> MGPVTINNFNYNDPIDNNNIIMMEPPFARGTGRYYKAFKITDRIWIIPERYTFGYKPEDFNKSSGIFNRDVCEYYDPDYLNTNDKKNIFLQTMIKLFNRIKSKPLGEKLLEMIINGIPYLGDRRVPLEEFNTNIASVTVNKLISNPGEVERKKGIFANLIIFGPGPVLNENETIDIGIQNHFASREGFGGIMQMKFCPEYVSVFNNVQENKGASIFNRRGYFSDPALILMHQLIYVLHGLYGIKVDDLPIVPNEKKFFMQSTDAIQAEELYTFGGQDPSIITPSTDKSIYDKVLQNFRGIVDRLNKVLVCISDPNININIYKNKFKDKYKFVEDSEGKYSIDVESFDKLYKSLMFGFTETNIAENYKIKTRASYFSDSLPPVKIKNLLDNEIYTIEEGFNISDKDMEKEYRGQNKAINKQAYEEISKEHLAVYKIQMCKSVKAPGICIDVDNEDLFFIADKNSFSDDLSKNERIEYNTQSNYIENDFPINELILDTDLISKIELPSENTESLTDFNVDVPVYEKQPAIKKIFTDENTIFQYLYSQTFPLDIRDISLTSSFDDALLFSNKVYSFFSMDYIKTANKVVEAGLFAGWVKQIVNDFVIEANKSNTMDKIADISLIVPYIGLALNVGNETAKGNFENAFEIAGASILLEFIPELLIPVVGAFLLESYIDNKNKIIKTIDNALTKRNEKWSDMYGLIVAQWLSTVNTQFYTIKEGMYKALNYQAQALEEIIKYRYNIYSEKEKSNINIDFNDINSKLNEGINQAIDNINNFINGCSVSYLMKKMIPLAVEKLLDFDNTLKKNLLNYIDENKLYLIGSAEYEKSKVNKYLKTIMPFDLSIYTNDTILIEMFNKYNSEILNNIILNLRYKDNNLIDLSGYGAKVEVYDGVELNDKNQFKLTSSANSKIRVTQNQNIIFNSVFLDFSVSFWIRIPKYKNDGIQNYIHNEYTIINCMKNNSGWKISIRGNRIIWTLIDINGKTKSVFFEYNIREDISEYINRWFFVTITNNLNNAKIYINGKLESNTDIKDIREVIANGEIIFKLDGDIDRTQFIWMKYFSIFNTELSQSNIEERYKIQSYSEYLKDFWGNPLMYNKEYYMFNAGNKNSYIKLKKDSPVGEILTRSKYNQNSKYINYRDLYIGEKFIIRRKSNSQSINDDIVRKEDYIYLDFFNLNQEWRVYTYKYFKKEEEKLFLAPISDSDEFYNTIQIKEYDEQPTYSCQLLFKKDEESTDEIGLIGIHRFYESGIVFEEYKDYFCISKWYLKEVKRKPYNLKLGCNWQFIPKDEGWTEHHHHHHHHHH;> MNINDNLSINSPVDNKNVVVVRARKTDTVFKAFK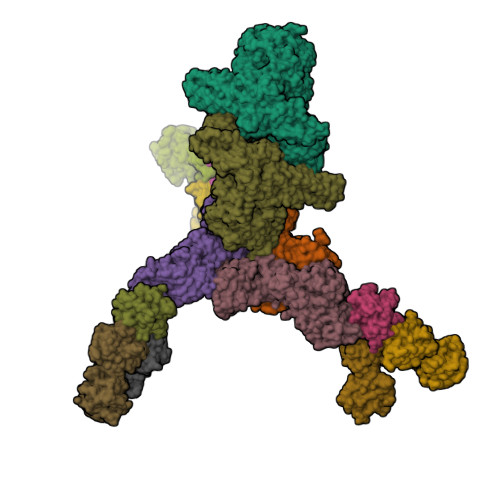VAPNIWVAPERYYGESLSIDEEYKVDGGIYDSNFLSQDSEKDKFLQAIITLLKRINSTNAGEKLLSLISTAIPFPYGYIGGGYYAPNMITFGSAPKSNKKLNSLISSTIPFPYAGYRETNYLSSEDNKSFYASNIVIFGPGANIVENNTVFYKKEDAENGMGTMTEIWFQPFLTYKYDEFYIDPAIELIKCLIKSLYFLYGIKPSDDLVIPYRLRSELENIEYSQLNIVDLLVSGGIDPKFINTDPYWFTDNYFSNAKKVFEDHRNIYETQIEGNNAIGNDIKLRLKQKFRININDIWELNLNYFSKEFSIMMPDRFNNALKHFYRKQYYKIDYPENYSINGFVNGQINVQLSLSDRNQDIINKPEEIINLLNGNNVSLMRSNIYGDGLKSTVDDFYSNYKIPYNRAYEYHFNNSNDSSLDNVNIGVIDNIPEIIDVNPYKENCDKFSPVQKITSTREINTNIPWPINYLQAQNTNNEKFSLSSDFVEVVSSKDKSLVYSFLSNVMFYLDSIKDNSPIDTDKKYYLWLREIFRNYSFDITATQEINTDCGINKVVTWFGKALNILNTSDSFVEEFQNLGPISLINKKENLSMPIIEIYGIPNDMLGLPLNDLNEKLFNIYLKNILYFKKVYFNFLDQWWTEYYSQYFDLICMAKQSILAQEKLIKQIIQNKLQDLFKADISMDKLNLMNLATEKTFIDLSNESQIAINNINDFLNKSAICVFDTNIYPKFISFMEQCINSVNSNVTAFIQKCTNITEDEKLQLIKLNTFMNIDFEFFDIQSIKDLITSETDLIKEEKESDYNLFLFTLQEDNNKVIEDISGKNTLVKYSDSISLVYGVNGDALYLKEPDESVSFSNKAFENGLTNSFSICFWLRNLGEDIITSKLIENKADNCGWEIYFENNGLVFSIVDCNGNEENIYLSDVISKNWYYISISIDRLRNQLLIFINDKLIANQSIEQILNIYSSNTISLVNENNPIYIEGLSILNRSITSEEVVNNYFSYLNNSYIRDISGERLEYNKTYELYNYVFPENSLYEVTENNNIYLSIKDTNNLNIQGAKFKLINIDANKQYVQKWDEGVVCLLGDEEKYVDISSENNRIQLVNSKDTAKRIIFNNDIFMPNCLTFAYNNKYLSLSLRDRNYNWMICNNNDNIPKAAHLWALKGI;>[3x]MNSSIKKIYNHIQEKVINYSDTIDLADGNYVVSRGDGWILSRQNQILGGSVISNGSTGIVGDLRVNDNAIPYYYPTPSFNEEYIKNNIQTVFANFTEANQIPIGFEFSKTAPSNKNLYMYLQYTYIRYEIIKVLQHEIIERAVLYVPSLGYVKSIEFNPGEKINKDFYFLTNDKCILNEQFLYKKILETTKNIPTNNIFNSKVSSTQRVLPYSNGLYVINKGDGYIRTNDKDLIGTLLIEAGSSGSIIQPRLRNTTRPLFTTSNDAKFSQQYTEERLKDAFNVQLFNTSTSLFKFVEEAPSNKNICIKAYNTYEKYELIDYQNGSIVNKAEYYLPSLGYCEVTNAPSPESEVVKTQVAEDGFIQNGPEEEIVVGVIDPSENIQEINTAISDNYTYNIPGIVNNNPFYILFTVNTTGIYKINAQNNLPSLKIYEAIGSGNRNFQSGNLCDDDIKAINYITGFDSPNAKSYLVVLLNKDKNYYIRVPQTSSNIENQIKFKREEGDLRNLMNSSVNIIDNLNSTGAHYYTRQSPDVHDYISYEFTIPGNFNNKDTSNIRLYTSYNQGIGTLFRVTETIDGYNLINIQQNLNLLNSTKSIRLLNGAIYILKVEVTELNNYNIKLHIDITN;>[3x]MSAERTFLPNGNYNIKSIFSGSLYLSPVSGSLTFSNESSANNQKWNVEYMAENRCFKISNVAEPNKYLSYDNFGFISLDSLSNRCYWFPIKIAVNTYIMLSLNKVNELDYAWDIYDTNENILSQPLLLLPNFDIYNSNQMFKLEKI;>[6x]MEHYSTIQNSLNDKIVTISCKANTDLFFYQVPGNGNVSLFQQTRNYLERWRIIYDSNKAAYKIKSMNIYNTNLVLTWNAPTHNISAQQDSNADNQYWLLLKDIGNNSFIIASYKNPNLVLYADTVARNLKLSTLNNSSYIKFIIEDYVISDFKNFTCRISPILAGGKVVQQVSMTNLAVNLYIWNNDLNQKWTIIYNEEKAAYQFFNKILSNGVLTWIFSDGNTVRVSSSAQNNDAQYWLINPVSDNYDRYTITNLRDKTKVLDLYGGQTADGTTIQVFNSNGGDNQIWTMSNP> MAFELPNLPYGFRALEPHIDQQTMEIHHDKHHNTYVTKLNAAVEGTDLESKSIEE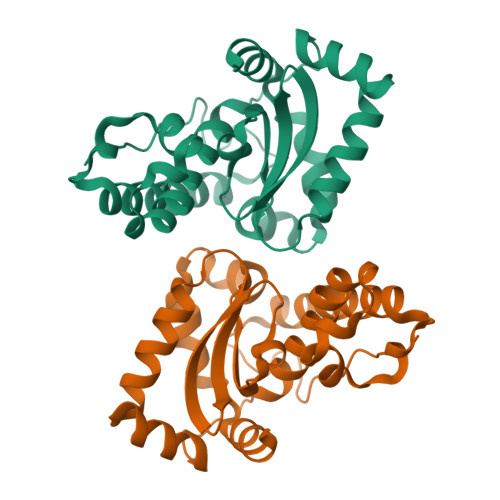IVANLDSVPENIQTAVRNNGGGHLNHSLFWELLTPNSEEKGTVVDKIKEQWGSLDAFKEEFANQAAARFGSGWAWLVVNDGKLEIVTTPNQDNPLTEGKTPILGLDVWEHAYYLKYQNKRPDYISAFWNVVNWEKVDELYNAAK>MAAQKSPQDMDRFIDALMKKMTVEEKIGQLNLPVTGEITTGQAKSSDIAAKIKRGEVGGLFNLKGVEKIRDVQKQAVEQSRLGIPLLFGMDVIHGYETMFPIPLGLSCTWDMTAIEESARIAAIEASADGISWTFSPMVDISRDPRWGRVSEGSGEDPFLGAMIAEAMVLGYQGKDMQRNDEIMACVKHFALYGAGEGGRDYNTVDMSRQRMFNEYMLPYEAAVEAGVGSVMASFNEVDGVPATANKWLMTDVLRGQWGFNGFVVTNYTGISEMIDHGIGDLQTVSARAINAGVDMDMVSEGFVSTLKKSIQEGKVSMETLNTACRRILEAKYKLGLFDNPYKYCDLKRPARDIFTKAHRDAARRIAAESFVLLKNDNVTLRPGTPAEPLLPFNPKGNIAVIGPLADSRTNMPGTWSVAAVLDRCPSLVEGLKEMTAGKANILYAKGSNLISDASYEERATMFGRSLNRDNRTDEQLLNEALTVANQSDIIIAALGESSEMSGESSSRTDLNIPDVQQNLLKELLKTGKPVVLVLFTGRPLTLTWEQEHVPAILNVWFGGSEAAYAIGDALFGYVNPGGKLTMSFPKNVGQIPLYYAHKNTGRPLAQGKWFEKFRSNYLDVDNEPLYPFGYGLSYTTFSYGD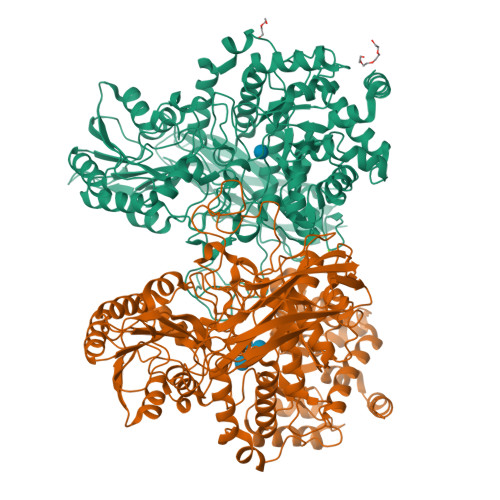IDLSRSTIDMTGELTAAVMVTNTGTWPGSEVVQLYIRDLVGSTTRPVKELKGFQKIFLEPGQSEIVRFKIAPEMLRYYNYDLQLVAEPGEFEVMIGTNSRDVKSARFTLKLEHHHHHH[2x]> MDITVREHDFKHGFIKSNSTFDGLNIDNSKNKKKIQKGFQILYVLLFCSVMCGLFYYVYENVWLQRDNEMNEILKNSEHLTIGFKVENAHDRILKTIKTHKLKNYIKESVNFLNSGLTKTNYLGSSNDNIELVDFQNIMFYGDAEVGDNQQPFTFI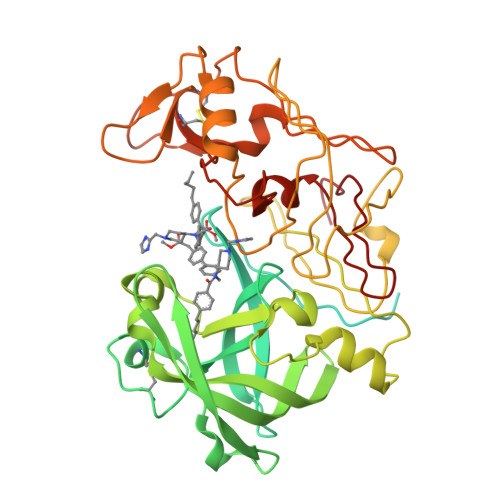LDTGSANLWVPSVKCTTAGCLTKHLYDSSKSRTYEKDGTKVEMNYVSGTVSGFFSKDLVTVGNLSLPYKFIEVIDTNGFEPTYTASTFDGILGLGWKDLSIGSVDPIVVELKNQNKIENALFTFYLPVHDKHTGFLTIGGIEERFYEGPLTYEKLNHDLYWQITLDAHVGNIMLEKANCIVDSGTSAITVPTDFLNKMLQNLDVIKVPFLPFYVTLCNNSKLPTFEFTSENGKYTLEPEYYLQHIEDVGPGLCMLNIIGLDFPVPTFILGDPFMRKYFTVFDYDNHSVGIALAKKNL4-(2-{(4M)-4-[(6M)-6-(2,5-dimethoxyphenyl)pyridin-3-yl]-1H-1,2,3-triazol-1-yl}ethyl)-N,N-dimethylbenzamide | C26 H27 N5 O3 | 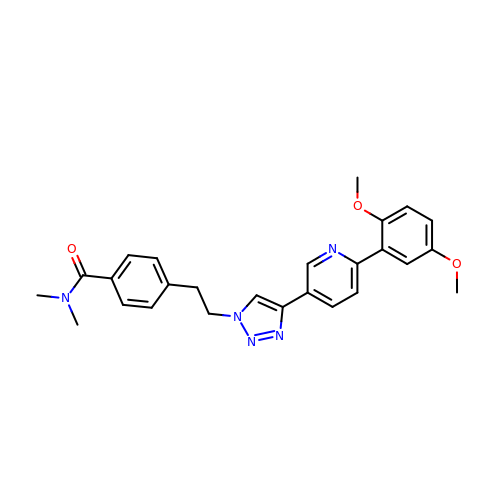IWENWSLJIVZDTH-UHFFFAOYSA-N> ADTIVAVELDSYPNTDIGDPNYPHIGIDIKSIRSKSTARWNMQTGKVGTVHISYNSVAKRLSAVVSYSGSSSTTVSYDVDLNNVLPEWVRVGLSATTGLYKETNTILSWSFTSKLKTNSAADENSLHFSFHKFSQNPKDLILQGDAFTDSDGNLELTKVSSSGDPQGNSVGRALFYAPVHIWEKSAVVASFDATFTF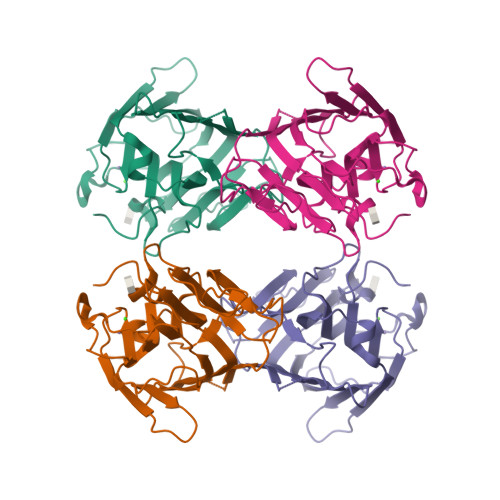LIKSPDREPADGITFFIANTDTSIPSGSGGRLLGLFPDAN>[30x]MSMYTTAQLLAANEQKFKFDPLFLRLFFRESYPFTTEKVYLSQIPGLVNMALYVSPIVSGEVIRSRGGSTSEFTPGYVKPKHEVNPQMTLRRLPDEDPQNLADPAYRRRRIIMQNMRDEELAIAQVEEMQAVSAVLKGKYTMTGEAFDPVEVDMGRSEENNITQSGGTEWSKRDKSTYDPTDDIEAYALNASGVVNIIVFDPKGWALFRSFKAVKEKLDTRRGSN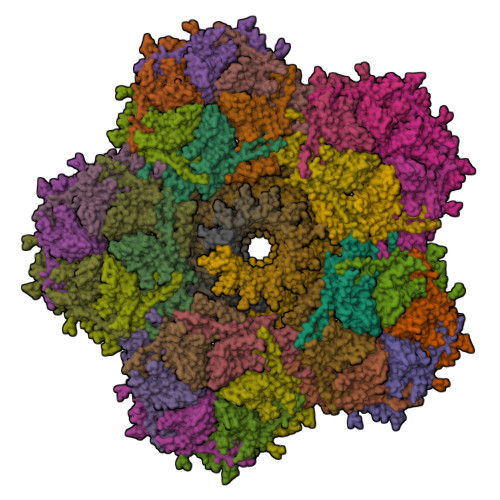SELETAVKDLGKAVSYKGMYGDVAIVVYSGQYVENGVKKNFLPDNTMVLGNTQARGLRTYGCIQDADAQREGINASARYPKNWVTTGDPAREFTMIQSAPLMLLADPDEFVSVQLA;>MKTPTIPTLLGPDGMTSLREYAGYHGGGSGFGGQLRSWNPPSESVDAALLPNFTRGNARADDLVRNNGYAANAIQLHQDHIVGSFFRLSHRPSWRYLGIGEEEARAFSREVEAAWKEFAEDDCCCIDVERKRTFTMMIREGVAMHAFNGELFVQATWDTSSSRLFRTQFRMVSPKRISNPNNTGDSRNCRAGVQINDSGAALGYYVSEDGYPGWMPQKWTWIPRELPGGRASFIHVFEPVEDGQTRGANVFYSVMEQMKMLDTLQNTQLQSAIVKAMYAATIESELDTQSAMDFILGANSQEQRERLTGWIGEIAAYYAAAPVRLGGAKVPHLMPGDSLNLQTAQDTDNGYSVFEQSLLRYIAAGLGVSYEQLSRNYAQMSYSTARASANESWAYFMGRRKFVASRQASQMFLCWLEEAIVRRVVTLPSKARFSFQEARSAWGNCDWIGSGRMAIDGLKEVQEAVMLIEAGLSTYEKECAKRGDDYQEIFAQQVRETMERRAAGLKPPAWAAAAFESGLRQSTEEEKSDSRAA[12x]DIETHYLCARBAMODITHIOIC ACID | C5 H11 N S2 | 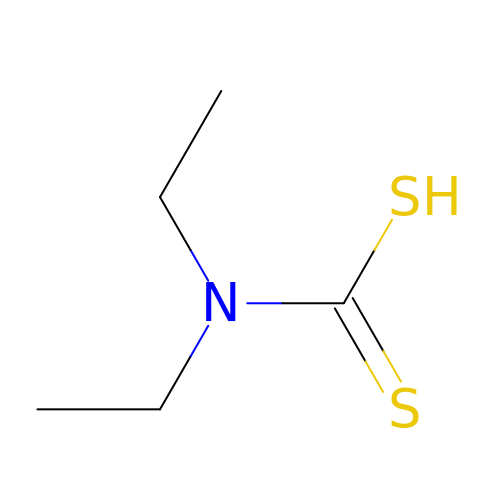LMBWSYZSUOEYSN-UHFFFAOYSA-N>[2x]MMNPSHGRGLGSAGGSSSGRNQGGGGETVVEMFPSGLRVLVVDDDPTCLMILERMLRTCLYEVTKCNRAEMALSLLRKNKHGFDIVISDVHMPDMDGFKLLEHVGLEMDLPVIMMSADDSKSVVLKGVTHGAVDYLIKPVRMEALKNIWQHVVRKRRSEWSVPEHSGSIEETGERQQQQHRGGGGGAAVSGGEDAVDDNSSSVNEGNNWRSSSRKRKDEEGEEQGDDKDEDASNLKKPRVVWSVEL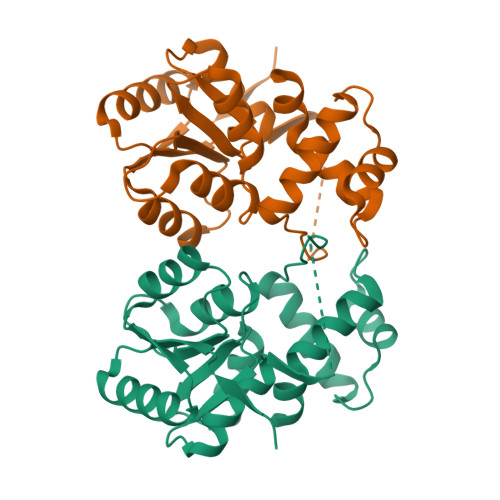HQQFVAAVNQLGVEKAVPKKILELMNVPGLTRENVASHLQKYRIYLRRLGGVSQH> MASLSRFRGCLAGALLGDCVGSFYEAHDTVDLTSVLRHVQSLEPDPGTPGSERTEALYYTDDTAMARALVQSLLAKEAFDEVDMAHRFAQEYKKDPDRGYGAGVVTVFKKLLNPKCRDVFEPARAQFNGKGSYGNGGAMRVAGISLAYSSVQDVQKFARLSAQLTHASSLGYNGAILQALAVHLALQGESSSEHFLKQLLGHMEDLEGDAQSVLDARELGMEERPYSSRLKKIGELLDQASVTREEVVSELGNGIAAFESVP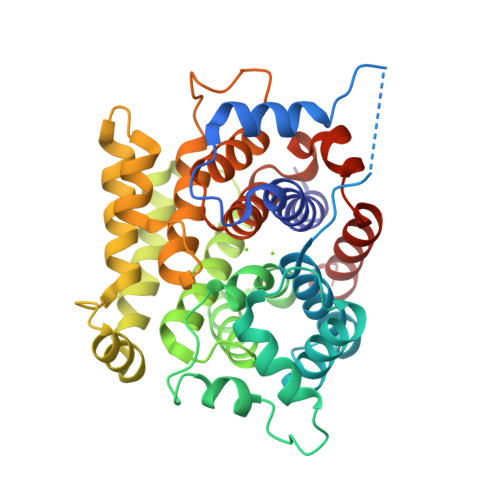TAIYCFLRCMEPDPEIPSAFNSLQRTLIYSISLGGDTDTIATMAGAIAGAYYGMDQVPESWQQSCEGYEETDILAQSLHRVFQKS To extend the structural coverage of proteins with uncharacterized biological function, we targeted Pfam protein family Pfam06938 (DUF1285), for which we determined the structures of two representative members. The first structural representatives of the DUF1285 family revealed a novel fold consisting of repeated motifs. The structures revealed a conserved core with domain duplication and a superficial similarity of the C-terminal domain to pleckstrin homology-like folds. The conservation of the domain interface indicates a potential binding site that is likely to involve a nucleotide-based ligand, with genome-context and gene-fusion analyses additionally supporting a role for this family in signal transduction, possibly during oxidative stress.

The Sbal_2486 gene of Shewanella baltica OS155, a psychrotropic marine γ-proteobacterium, encodes a protein with a molecular weight of 17.7 kDa (residues 1–157) and a calculated iso­electric point of 4.8. The crystal structure of Sbal_2486 was determined to 1.4 Å resolution using the MAD method. The final model included a monomer of 127 residues, seven ethylene glycol molecules, one sodium ion and 231 water molecules in the asymmetric unit. No electron density was observed for residues Gly0 (which remained at the N-­terminus after cleavage of the purification tag), Gln9–Cys28 and Glu156–Gln157. The two domains of Sbal_2486 (residues 29–84 and 85–155) show close structural similarity to SPO0140 (Cα r.m.s.d. of 2.8 Å over 127 residues with a sequence identity of 25%). Thus, although the β3αβ3 repeat described for SPO0140 is present in the N-terminal domain of Sbal_2486, the loss of the C-terminal meander results in a truncated version of this repeat in the second domain. Sbal_2486 crystallized with one monomer in the asymmetric unit and PISA again suggested a monomer as the most probable oligomeric form. The largest packing interface buries ∼760 Å2 of solvent-accessible surface area but is not predicted to be stable for complex formation. However, the results of anSEC coupled with static light scattering (SLS) for Sbal_2486 indicate a dimeric form in solution under the test conditions. This suggests that either the observed crystal-packing interface is stable or the oligomerization state is dependent on the buffer conditions, forming a dimer in the anSEC buffer but disassociating in the crystallization solution prior to crystal formation.

> GQHTLKQFAADSALTTTTPLCSEVPLFDINALGDWTYLGTSLPAKFAKLFASILHCIDDEYFLITPVEKVRVQVEDAPLLIVDFERAQPHSLLNVSTSIGTLHHNVDIKQMKLTDDSVYLPLERGLWGKLGRACYYNFVNEFNLSDLNEQ> MLEQPYLDLAKKVLDEGHFKPDITHTGTYSIFGHQMRFDLSKGFPLLTTKKVPFGLIKSELLWFLHGDTNIRFLLQHRNHIWDEWAFEKWVKSDEYHGPDMTDFGHRSQKDPEFAAVYHEEMAKFDDRVLHDDAFAAKYGDLGLVYGSQWRAWHTS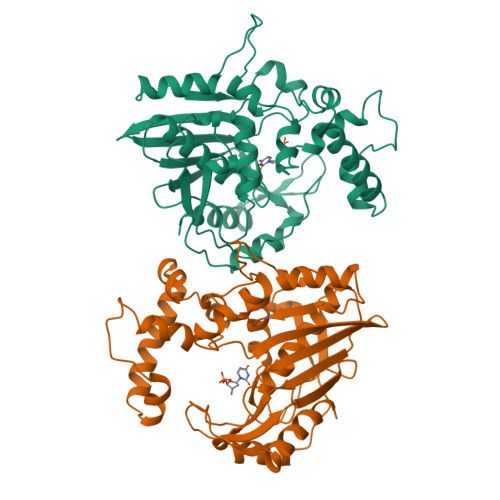KGDTIDQLGDVIEQIKTHPYSRTLIVSAWNPEDVPTMALPPCHTLYQFYVNDGKLSLQLYQRSADIFLGVPFNIASYALLTHLVAHECGLEVGEFIHTFGDAHLYVNHLDQIKEQLSRTPRPAPTLQLNPDKHDIFDFDMKDIKLLNYDPYPAIKAPVAV N~2~-[(2R)-4-(HYDROXYAMINO)-2-(2-NAPHTHYLMETHYL)-4-OXOBUTANOYL]-L-ARGINYLGLYCYLGLYCINAMIDE | C25 H34 N8 O6 | 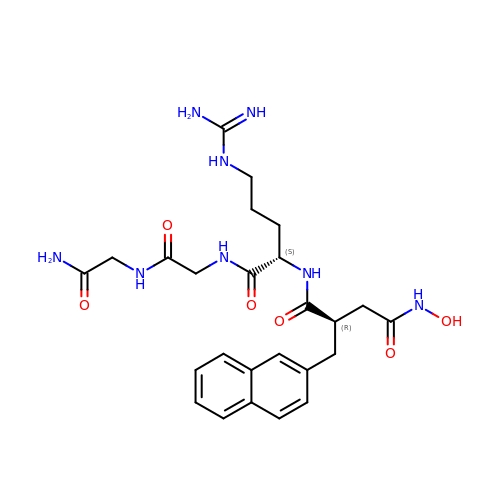NINUSDCYEXCHSI-MOPGFXCFSA-N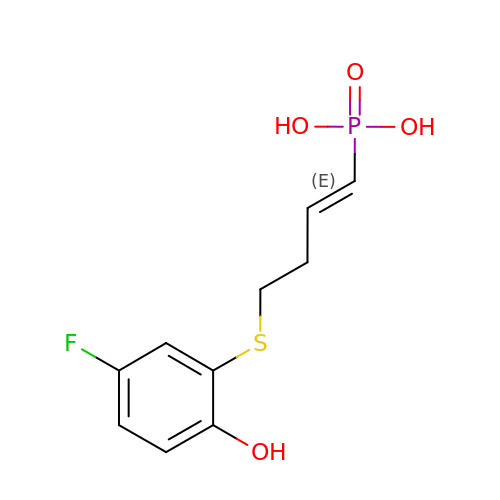4-(2-HYDROXY-4-FLUOROPHENYLTHIO)-BUTYLPHOSPHONIC ACID | C10 H12 F O4 P S | UXOYJQMPYTYCMG-ORCRQEGFSA-N>[2x]MNVDEFLFISNNFKQYKEFIDMDTAKHYFECRNIEGLNHILDSYKDSKSTKEKNL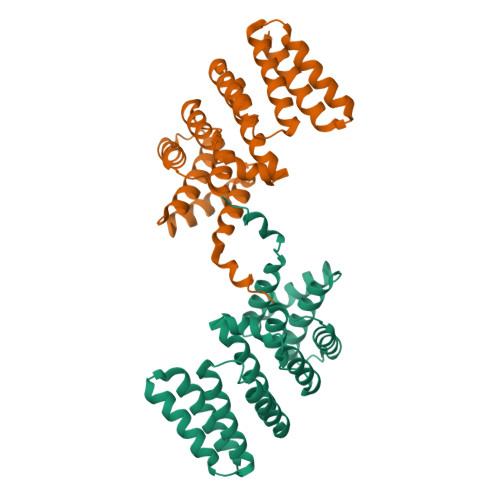FALVKVLLATLTEEDCLTERTYLSNYLINIETWSHYETVLFNNCMFIFESCFIEMVFSKVILNLDKYNTLRYYGNESIRMFVNMLILFIQRQEYDKASEILAKIEDYQLNDDCLYERCCVSFFDGIIGLINGKEGAEQKCVQILEIFQLLNCKTIHHMFQTYLEAIKHKLSLEHHHHHH>DYNHWLIVMEFPKDPAPSRDQMIDTYLNTLATVLGSMEEAKKNMYAFSTTTYTGFQCTIDEETSEKFKGLPGV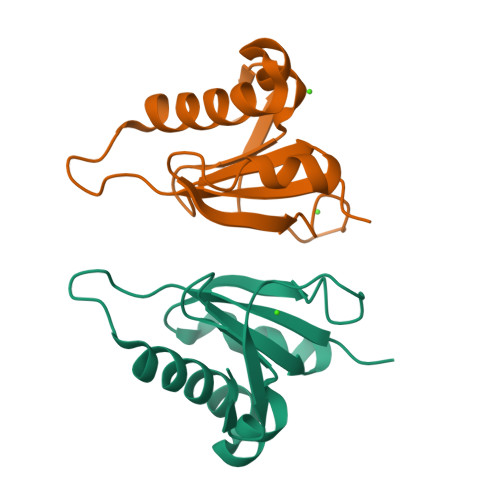LWVLPDSYIDVKNKDYGGDKYINGEIIP[2x]(3-(2-FLUOROPHENYL)-N-(1-(2-OXO-2,3-DIHYDRO-1H-BENZO[D]IMIDAZOL-5-YL)ETHYL)BUTANAMIDE) 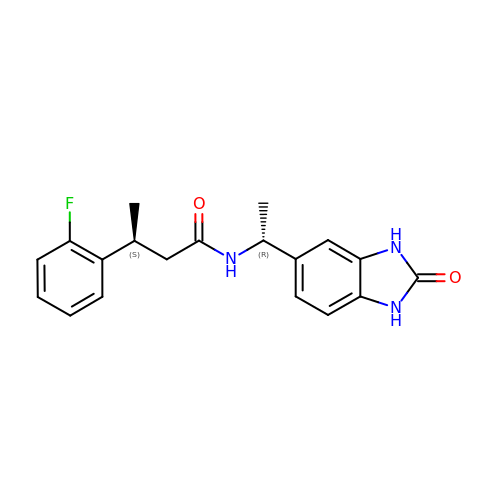| C19 H20 F N3 O2 | QMZGJDIRPYTWRL-NWDGAFQWSA-N> SEESQAFQRQLTALIGYDVTDVSNVHDDELEFTRRGLVTPRMAEVASRDPKLYAMHPWVTSKPLPEYLWKKIANNCIFIVIHRSTTSQTIKVSPDDTPGAILQSFFTKMAKKKSLMDIPESQSEQDFVLRVCGRDEYLVGETPIKNFQWVRHCLKNGEEIHVVLDTPPDPALDEVRKEEWPLVDDCTGVTGYHEQLTIHGKDHESVFTVSLWDCDRKFRVKIRGIDIPVLPRNTDLTVFVEANIQHGQQVLCQRRTSPKPFTEEVLWNVWLEFSIKIKDLPKGALLNLQIYCGKAPALSSKASAESPSSESKGKVQLLYYVNLLLIDHRFLLRRGEYVLHMWQISGKGEDQGSFNADKLTSATNPDKENSMSISILLDNYCHPIALPKHQPTPDPEGDRVRAEMPNQLRKQLEAIIATDPLNPLTAEDKELLWHFRYESLKHPKAYPKLFSSVKWGQQEIVAKTYQLLARREVWDQSALDVGLTMQLLDCNFSDENVRAIAVQKLESLEDDDVLHYLLQLVQAVKFEPYHDSALARFLLKRGLRNKRIGHFLFWFLRSEIAQSRHYQQRFAVILEAYLRGCGTAMLHDFTQQVQVIEMLQKVTLDIKSLSAEKYDVSSQVISQLKQKLENLQNSQLPESFRVPYDPGLKAGALAIEKCKVMASKKKPLWLEFKCA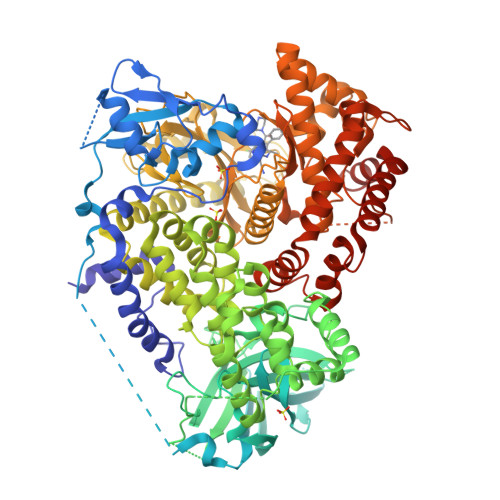DPTALSNETIGIIFKHGDDLRQDMLILQILRIMESIWETESLDLCLLPYGCISTGDKIGMIEIVKDATTIAKIQQSTVGNTGAFKDEVLNHWLKEKSPTEEKFQAAVERFVYSCAGYCVATFVLGIGDRHNDNIMITETGNLFHIDFGHILGNYKSFLGINKERVPFVLTPDFLFVMGTSGKKTSPHFQKFQDICVKAYLALRHHTNLLIILFSMMLMTGMPQLTSKEDIEYIRDALTVGKNEEDAKKYFLDQIEVCRDKGWTVQFNWFLHLVLGIKQGEKHSA> MNEQRSVAVWRDGAAVTVPAHQPVVTAFDLGLGRGDGIFESVAVVAGRTPHLAAHLTRLTRSAALLGLPAPGDQAWMEMVAAVLADWPAALEGVCRLFLTRGLGDGTPPTALALLAPVPADTLRQRAEGISVATLGLGVPADFRAGAPWLLGGAKTLSYAVNMAAQRHAHDLGADDVVFTSLEGRLLEGPTSTVVWAAGGTLHTPPVETGILPGTTQARLFTAAAADGWPTSVTPGTVDDLHAADAVWLLSGVRGAAVVHTVDGVRRGDGDLSRRVRELLA

Here, we analyze the structure–function relationships in a non-canonical D-amino acid transaminase from Blastococcus saxobsidens, which is active towards D-amino acids and primary (R)-amines. The catalytic unit of a TA is a homodimer with two active sites at the dimer interface, containing PLP covalently bound to the catalytic lysine. The organization of the functional dimer of BlasaTA is typical of PLP fold type IV TAs. We suggest that the features of the active site of transaminase from B. saxobsidens, such as the flexibility of the R34 and R96 residues, the lack of bulky residues in the β-turn at the entrance to the active site, and the short O-pocket loop, facilitate the binding of substrates with and without α-carboxylate groups.

A detailed study of the enzyme includes a kinetic analysis of its substrate scope and a structural analysis of the holoenzyme and its complex with phenylhydrazine—a reversible inhibitor and analogue of (R)-1-phenylethylamine—a benchmark substrate of (R)-selective amine transaminases. In the complex, the electron density in the active site corresponds to the mixture of the adduct of PLP and phenylhydrazine, mimicking the external aldimine, and an apoform of BlasaTA with equal occupancies. In the structure of the complex with phenylhydrazine, the linkage between phenylhydrazine and PLP is clearly observed in the electron density map, with a dihedral angle C3-C4-C4α-N of about 40°. The pyridine ring of the cofactor is tilted by 12° around the N1-C6 bond from its position in the holoenzyme. The released ε-NH2 group of K155 forms a hydrogen bond with the N4′ atom of the adduct. Notably, the accommodation of the phenyl ring in the O-pocket is accompanied by the formation of stacking interactions with the side chain of F39 and the removal of the side chains of residues R96 and R34* from the active site. The orientation of the D105* and D121 residues is slightly changed, resulting in the shortening of the distance between the oxygen atoms of γ-carboxylate groups from 12.3 Å in the holoenzyme to 11.00 Å in the complex. The RMSD for the Cα atoms between the subunits of the holoenzyme and the complex did not exceed 0.2 Å, indicating no gross structural changes upon substrate binding. The reaction between the PLP form of BlasaTA and phenylhydrazine was limited to the formation of the external aldimine (transimination step), whose accumulation was observed at 370 nm. According to the analysis of the crystal structures of the holoenzyme and the complex with phenylhydrazine, an analogue of the substrate (R)-1-phenylethylamine, the active site of BlasaTA, shares common features with another non-canonical DAAT of expanded substrate specificity from C. pusillum.>MAAGVAAWLPFARAAAIGWMPVASGPMPAPPRQERKRTQDALIVLNVSGTRFQTWQDTLERYPDTLLGSSERDFFYHPETQQYFFDRDPDIFRHILNFYRTGKLHYPRHECISAYDEELAFFGLIPEIIGDCCYEEYKDRRRENAERLQDDADTDTAGESALPTMTARQRVWRAFENPHTSTMALVFYYVTGFFIAVSVIANVVETVPCGSSPGHIKELPCGERYAVAFFCLDTACVMIFTVEYLLRLAAAPSRYRFVRSVMSIIDVVAILPYYIGLVMTDNEDVSGAFVTLRVFRVFRIFKFSRHSQGLRILGYTLKSCASELGFLLFSLTMAIIIFATVMFYAEKGSSASKFTSIPAAFWYTIVTMTTLGYGDMVPKTIAGKIFGSICSLSGVLVIALPVPVIVSNFSRIYHQNQRADKRRAQKKARLARIRAAKSGSANAYMQSKRSGLLSNQLQSSEDEPAFVSKSGSSFETQHHHLLHCLEKTTNHEFVDEQVFEESCMEVATVNRPSSHSPSLSSQQGVTSTCCSRRHKKTFRIPNANVSGSHRGSVQELSTIQIRCVERTPLSNSRSSLNAKMEECVKLNCEQPYVTTAIISIPTPPVTTPEGDDRPESPEYSGGNIVRVSAL[4x];>[4x]MGAVMGTFSSLQTKQRRPSKDKIEDELEMTMVCHRPEGLEQLEAQTNFTKRELQVLYRGFKNECPSGVVNEDTFKQIYAQFFPHGDASTYAHYLFNAFDTTQTGSVKFEDFVTALSILLRG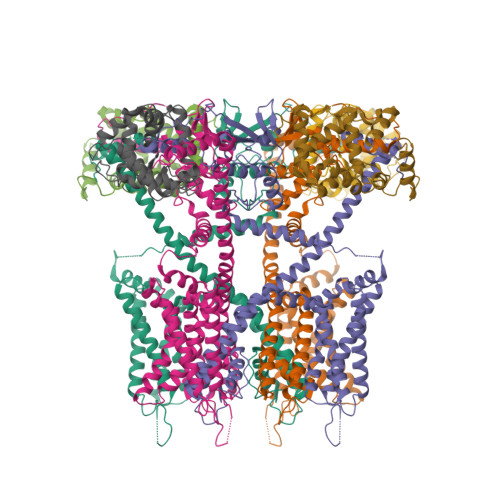TVHEKLRWTFNLYDINKDGYINKEEMMDIVKAIYDMMGKYTYPVLKEDTPRQHVDVFFQKMDKNKDGIVTLDEFLESCQEDDNIMRSLQLFQNVM>MHHHHHHSSGRENLYFQGTLGINGFGRIGRLVLRACMERNDITVVAINDPFMDVEYMAYLLKYDSVHGNFNGTVEVSGKDLCINGKVVKVFQAKDPAEIPWGASGAQIVCESTGVFTTEEKASLHLKGGAKKVIISAPPKDNVPMYVMGVNNTEYDPSKFNVISNASCTTNCLAPLAKIINDKFGIVEGLMTTVHSLTANQLTVDGPSKGGKDWRAGRCAGNNIIPASTGAAKAVGKVIPALNGKLTGMAIRVPTPDVSVVDLTCKLAKPASIEEIYQAVKEASNGPMK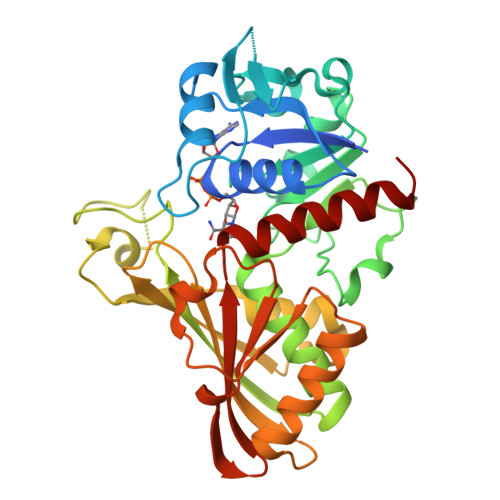GIMGYTSDDVVSTDFIGCKYSSIFDKNACIALNDSFVKLISWYDNESGYSNRLVDLAVYVASRGL[2x]>[2x]KTSDANETEDHLESLICKVGEKSACSLESNLEGLAGVLEADLPNYKSKILRLLCTVARLLPEKLTIYTTLVGLLNARNYNFGGEFVEAMIRQLKESLKANNYNEAVYLVRFLSDLVNCHVIAAPSMVAMFENFVSVTQEEDVPQVRRDWYVYAFLSSLPWVG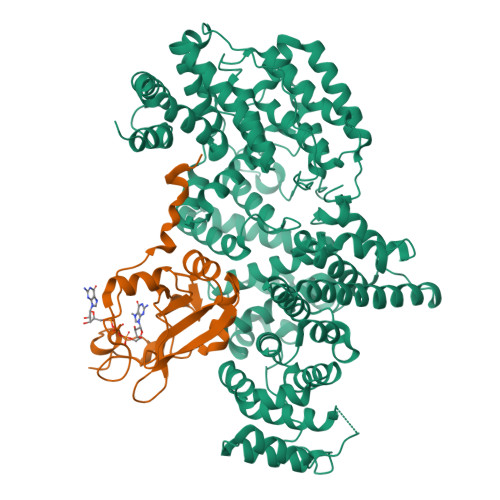KELYEKKDAEMDRIFANTESYLKRRQKTHVPMLQVWTADKPHPQEEYLDCLWAQIQKLKKDRWQERHILRPYLAFDSILCEALQHNLPPFTPPPHTEDSVYPMPRVIFRMFDYTDDPEGPVMPGSHSVERFVIEENLHCIIKSHWKERKTCAAQLVSYPGKNKIPLNYHIVEVIFAELFQLPAPPHIDVMYTTLLIELCKLQPGSLPQVLAQATEMLYMRLDTMNTTCVDRFINWFSHHLSNFQFRWSWEDWSDCLSQDPESPKPKFVREVLEKCMRLSYHQRILDIVPPTFSALCPSNPTCIYKYGDESSNSLPGHSVALCLAVAFKSKATNDEIFSILKDVPNPNQDDDDDEGFSFNPLKIEVFVQTLLHLAAKSFSHSFSALAKFHEVFKTLAESDEGKLHVLRVMFEVWRNHPQMIAVLVDKMIRTQIVDCAAVANWIFSSELSRDFTRLFVWEILHSTIRKMNKHVGAQSEQKNLFLVIFQRFIMILTEHLVRCETDGTSVLTPWYKNCIERLQQIFLQHHQIIQQYMVTLENLLFTAELDPHILAVFQQFCALQA;>[2x]MSGGLLKALRSDSYVELSQYRDQHFRGDNEEQEKLLKKSCTLYVGNLSFYTTEEQIYELFSKSGDIKKIIMGLDKMKKTACGFCFVEYYSRADAENAMRYINGTRLDDRIIRTDWDAGFKEGRQYGRGRSGGQVRDEYRQDYDAGRGGYGKLAQNQ>[2x]GSHMTKTITVAHIQYDFKAVLEENDENDD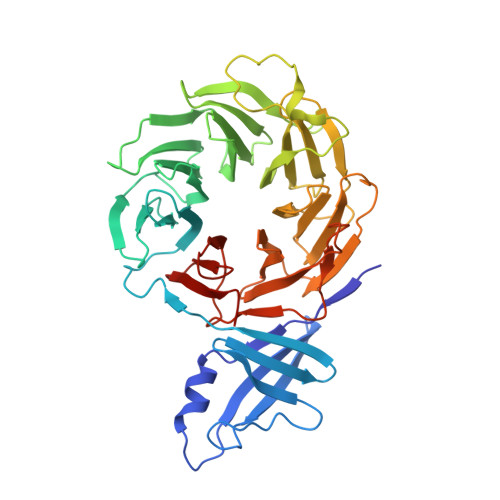EFYINVDKNLNEIKEHKIVVLGNSRGVDAGKGNTFEKVGSHLYKARLDGHDFLFNTIIRDGSKMLKRADYTAVDTAKLQMRRFILGTTEGDIKVLDSNFNLQREIDQAHVSEITKLKFFPSGEALISSSQDMQLKIWSVKDGSNPRTLIGHRATVTDIAIIDRGRNVLSASLDGTIRLWECGTGTTIHTFNRKENPHDGVNSIALFVGTDRQLHEISTSKKNNLEFGTYGKYVIAGHVSGVITVHNVFSKEQTIQLPSKFTCSCNSLTVDGNNANYIYAGYENGMLAQWDLRSPECPVGEFLINEGTPINNVYFAAGALFVSSGFDTSIKLDIISDPESERPAIEFETPTFLVSNDDAVSQFCYVSDDESNGEVLEVGKNNFCALYNLSNP>SMAENREPRGAVEAELDPVEYTLRKRLPSRLPRRPNDIYVNMKTDFKAQLARCQKLLDGGARGQNACSEIYIHGLGLAINRAINIALQLQAGSFGSLQVAANTSTVELVDELEPETDTREPLTRIRNNSAIHI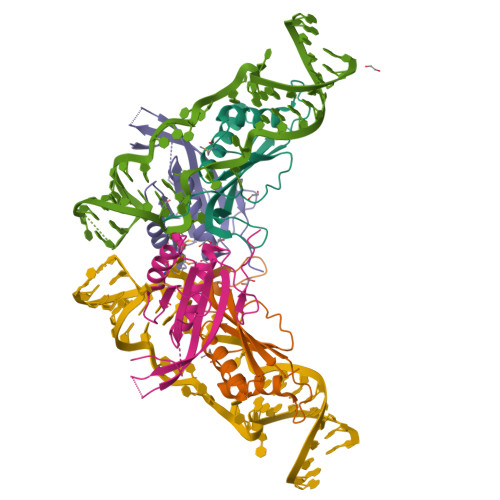RVFRVTPK[2x];>[2x]ENFRKVRSEEAPAGCGAEGGGPGSGPFADLAPGAVHMRVKEGSKIRNLMAFATASMAQPATRAIVFSGCGRATTKTVTCAEILKRRLAGLHQVTRLRYRSVREVWQSLPPGPTQGQTPGEPAASLSVLKNVPGLAILLSKDALDPRQPGYQPPNPHPGPSSPPAAPASKRSLGEPAAGEGSAKRSQPEPGVADEDQTA>[5x]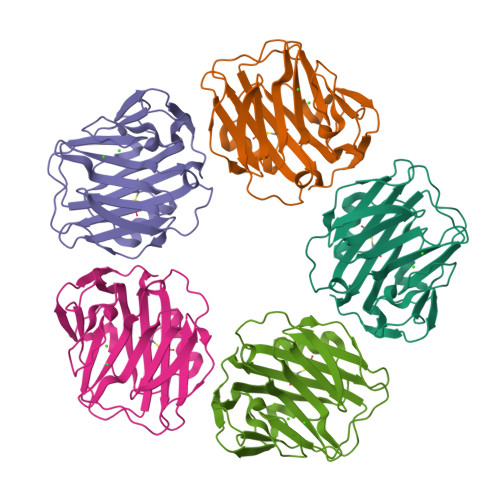QTDMSRKAFVFPKESDTSYVSLKAPLTKPLKAFTVCLHFYTELSSTRGYSIFSYATKRQDNEILIFWSKDIGYSFTVGGSEILFEVPEVTVAPVHICTSWESASGIVEFWVDGKPRVRKSLKKGYTVGAEASIILGQEQDSFGGNFEGSQSLVGDIGNVNMWDFVLSPDEINTIYLGGPFSPNVLNWRALKYEVQGEVFTKPQLWP>GQDMVSPPPPIADEPLTVNTGIYLIECYSLDDKAATFKVNAFLSLSWKDRRLAFDPVRSGVRVKTYEPEAIWIPEIRFVNVENARDADVVDISVSPDGTVQYLERFSARVLSPLDFRRYPFDSQTLHIYLIVRSVDTRNIVLAVDLEKVGKNDDVFLTGWDIESFTAVVKPANFALEDRLESKLDYQLRISRQYFSYIPNIILPMLFILFISWTAFWSTSYEANVTLVVSTLIAHIAFNILVETNLPKTPYMTYTGAIIFMIYLFYFVAVIEVTVQHYLKVESQPARAASITRASRIAFPVVFLLANIILA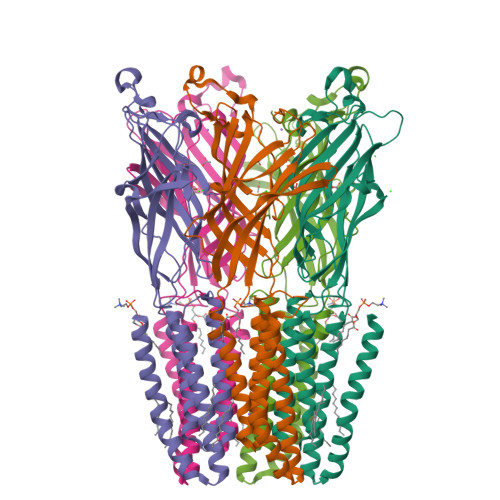FLFFGF[5x]We report an in silico strategy for the biocatalytic synthesis of chiral N- and O-heterocycles via Baldwin cyclization modes of hydroxy- and amino-substituted epoxides and oxetanes using the limonene epoxide hydrolase from Rhodococcus erythropolis. We turned to cofactor-independent limonene epoxide hydrolases (LEHs) that normally catalyze direct hydrolysis of epoxides by positioning and activating water at the active site. On the basis of the well-documented mechanism of ReLEH, a water molecular is positioned by H-bonds to N55 and Y53 while D132 abstracts a proton from the water, enabling a smooth nucleophilic attack on one of the substrate’s epoxide carbon center. We have rationally engineered the epoxide hydrolase ReLEH with construction of a general platform for Baldwin cyclization reactivity of hydroxy- and amino-epoxides and oxetanes.

Several hits with essentially eliminated WT hydrolytic activity were identified, including variants SZ532 (Y53L/N55P), SZ534 (Y53V/N55P), SZ609 (Y53I/N55A) and SZ611 (Y53F/N55A). Indeed, they enable Baldwin-type cyclization with little formation of undesired 1,2-diols. In the case of the double mutant SZ611 (Y53F/N55A), the formation of Baldwin product 2 is improved from 10% (WT) up to 78% (2:3 = 7.8). Compared to WT, the hydrolysis conversion is largely decreased from 99 to 46%. These results suggest that the substitutions Y53F and N55A of ReLEH can effectively break the water binding network, thereby endowing Baldwin cyclization reactivity. SZ611 assembles into a homodimer structure with four α-helices and five-strand β-sheets in each monomer, forming a cavity that serves as a deep substrate-binding pocket, in which a substituent of substrate 59 or of product 46 can occur without steric repulsion. Two other essential mutations, Y53F and N55A, have well-defined electron density maps that together expand the hydrophobic local space, thereby leading to the preference of intramolecular cyclization reactions.

>[4x]MHHHHHHTSKIEQPRWASKDSAAGAASTPDEKIVLEFMDALTSNDAAKLIEYFAEDTMFQAMPLPPAYGRDAVEQTLAGLFTVMSIDAVETFHIGSSNGLVYTERVDVLRALPTGKSYNLSILGVFQLTEGKITGWRDYFDLREFEEAVDLPLRG> MNITDIREQFPILHQQVNGHDLVYLDSAATSQKPRAVIETLDKYYNQYNSNVHRGVHTLGTRATDGYEGAREKVRKFINAKSMAEII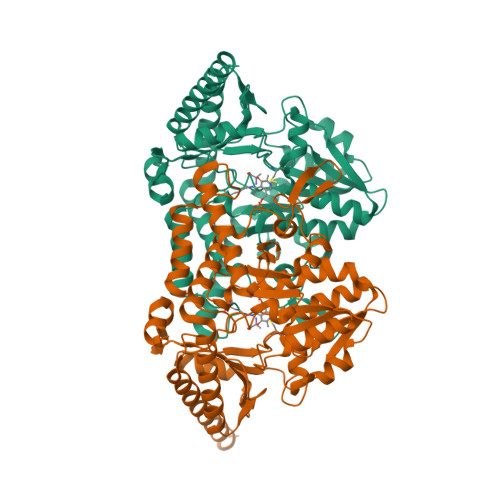FTKGTTTSLNMVALSYARANLKPGDEVVITYMEHHANIIPWQQAVKATGATLKYIPLQEDGTISLEDVRETVTSNTKIVAVSHVSNVLGTVNPIKEMAKIAHDNGAVIVVDGAQSTPHMKIDVQDLDCDFFALSSHKMCGPTGVGVLYGKKALLENMEPAEFGGEMIDFVGLYESTWKELPWKFEAGTPIIAGAIGLGAAIDFLEEIGLDEISRHEHKLAAYALERFRQLDGVTVYGPEERAGLVTFNLDDVHPHDVATVLDAEGIAVRAGHHCAQPLMKWLDVTATARASFYLYNTEEEIDKLVEALQKTKEYFTNVFSGHHHHHH> QETLVRPKPLLLKLLKSVGAQKDTYTMKEVLFYLGQYIMTKRLYDEKQQHIVYCSNDLLGDLFGVPSFSVKEHR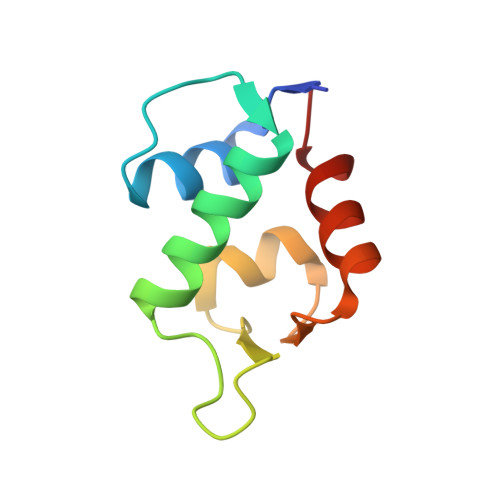KIYTMIYRNLVV> APLAQRVRIMGGTNRGRAEVYYNNEWGTICDDDWDNNDATVFCRMLGYSRGRALSSYGGGSGNIWLDNVNCRGTENSLWDCSKN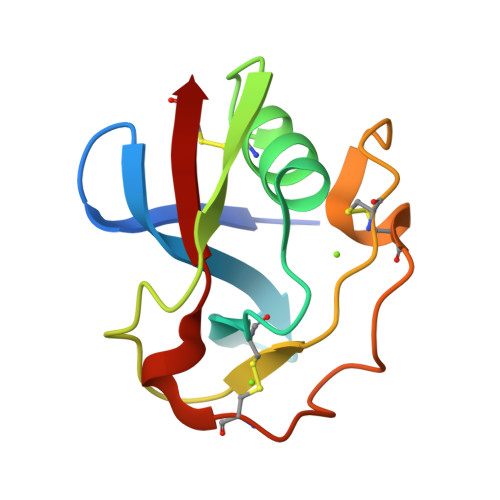SWGNHNCVHNEDAGVECS> GICSR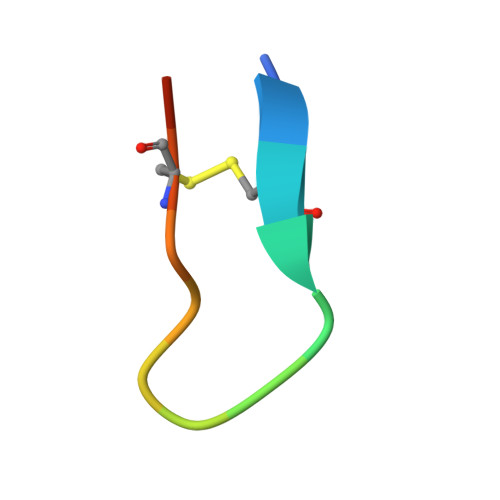SLPPICIPD> GAMAAGTL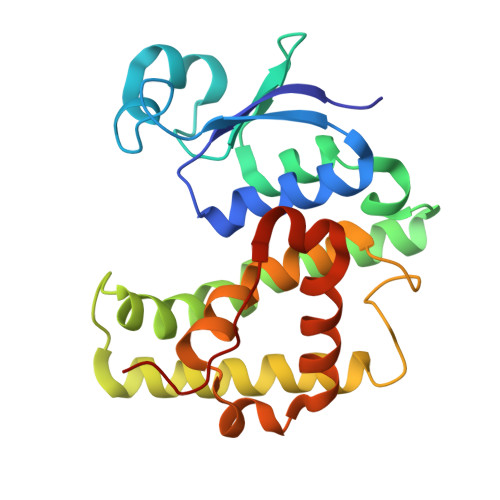YTYPENWRAFKALIAAQYSGAQVRVLSAPPHFHFGQTNRTPEFLRKFPAGKVPAFEGDDGFCVFESNAIAYYVSNEELRGSTPEAAAQVVQWVSFADSDIVPPASTWVFPTLGIMHHNKQATENAKEEVRRILGLLDAYLKTRTFLVGERVTLADITVVCTLLWLYKQVLEPSFRQAFPNTNRWFLTCINQPQFRAVLGEVKLCEKMAQFDA> SYFSAADVYVPDEWEVAREKITMSRELGQGSFGMVYEGVAKGVVKDEPETRVAIKTVNEAASMRERIEFLNEASVMKEFNCHHVVRLLGVVSQGQPTLVIMELMTRGDLKSYLRSLRPEMENNPVLAPPSLSKMIQMAGEIADGMAYLNANK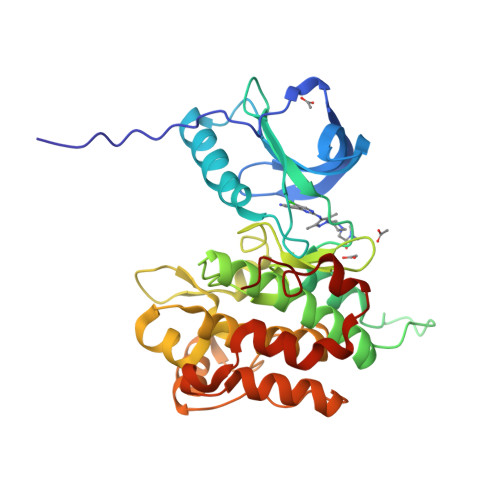FVHRDLAARNCMVAEDFTVKIGDFGMTRAIYETDYYRKGGKGLLPVRWMSPESLKDGVFTTYSDVWSFGVVLWEIATLAEEPYQGLSNEQVLRFVMEGGLLDKPDNCPDMLFELMRMCWQYNPKMRPSFLEIISSIKEEMEPGFREVSFYYSEENK>MRQVDAATHGGRAVIELREKILSGELPGGMRLFEVSTAELLDISRTPVREALSRLTEEGLLNRLPGGGFVVRRFGFADVVDAIEVRGVMEGTAARLAAERGVSKVALEEIDATVQQLDLCFGDRVDDVDFDGYAALNRIFHHQLAALCGSEMIRREVERASSLPFASPSAFLPDKANIGAFRRSLRGAQEQHKAIVAAIVAREGARAEAVAREHSRTARTNLEYMIREAPEL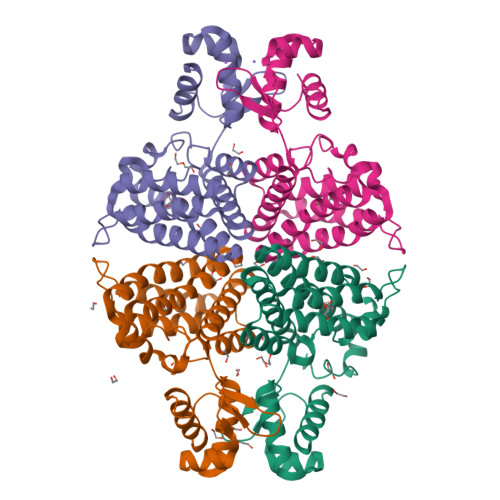IAQVPGLALISDHHHHHH[4x]> GPLEDQEENTLRELRLFLRDVTKRLATDKRFNIFSKPVDIEEVSDYLEVIKEPMDLSTVITKIDKHNYLTAKDFLKDIDLICSNALEYNPDKDPGDKI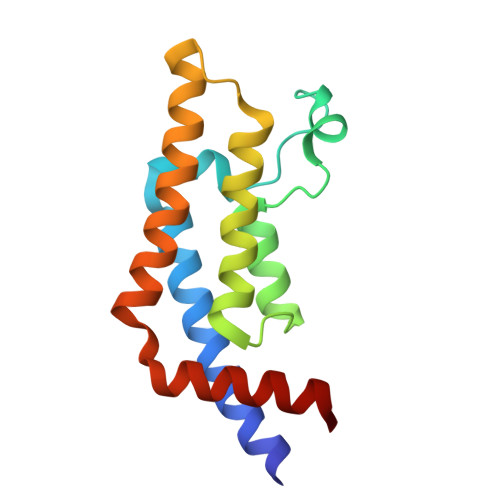IRHRACTLKDTAHAIIAAELDPEFNKLCEEIKEARIKR> GPASQHFLSTSVQGPWERAISPN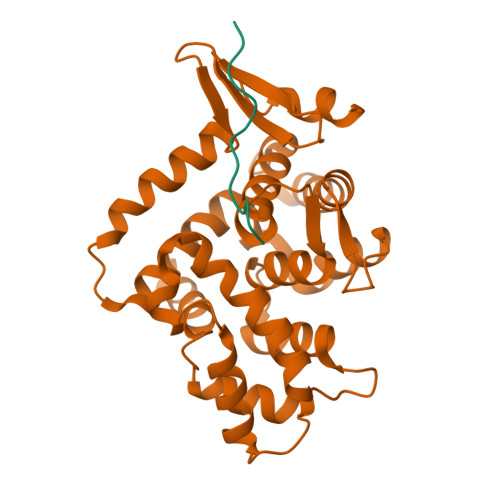KVPYYINHETQTTCWDHPKMTELYQSLADLNNVRFSAYRTAMKLRRLQKALCLDLLSLSAACDALDQHNLKQNDQPMDILQIINCLTTIYDRLEQEHNNLVNVPLCVDMCLNWLLNVYDTGRTGRIRVLSFKTGIISLCKAHLEDKYRYLFKQVASSTGFCDQRRLGLLLHDSIQIPRQLGEVASFGGSNIEPSVRSCFQFANNKPEIEAALFLDWMRLEPQSMVWLPVLHRVAAAET;> KNMTPYRSPPPYVPP>MSQHNEKNPHQHQSPLHDSSEAKPGMDSLAPEDGSHRPAAEPTPPGAQPTAPGSLKAPDTRNEKLNSLEDVRKGSENYALTTNQGVRIADDQNSLRAGSRGPTLLEDFILREKITHFDHERIPERIVHARGSAAHGYFQPYKSLSDITKADFLSDPNKITPVFVRFSTVQGGAGSADTVRDIRGFATKFYTEEGIFDLVGNNTPIFFIQDAHKFPDFVHAVKPEPHWAIPQGQSAHDTFWDYVSLQPETLHNVMWAMSDRGIPRSYRTMEGFGIHTFRLINAEGKATFVRFHWKPLAGKASLVWDEAQKLTGRDPDFHRRELWEAIEAGDFPEYELGFQLIPEEDEFKFDFDLLDPTKLIPEELVPVQRVGKMVLNRNPDNFFAENEQAAFHPGHIVPGLDFTNDPLLQGRLFSYTDTQISRLGGPNFHEIPINRPTCPYHNFQRDGMHRMGIDTNPANYEPNSINDNWPRETPPGPKRGGFESYQERVEGNKVRERSPSFGEYYSHPRLFWLSQTPFEQRHIVDGFSFELSKVVRPYIRERVVDQLAHIDLTLAQAVAKNLGIELTDDQLNITPPPDVNGLKKDPSLSLYAIPDGDVKGRVVAILLNDEVRSADLLAILKALKAKGVHAKLLYSRMGEVTADDGTVLPIAATFAGAPSLTVDAVIVPCGNIADIADNGDANYYLMEAYKHLKPIALAGDARKFKATIKIADQGEEGIV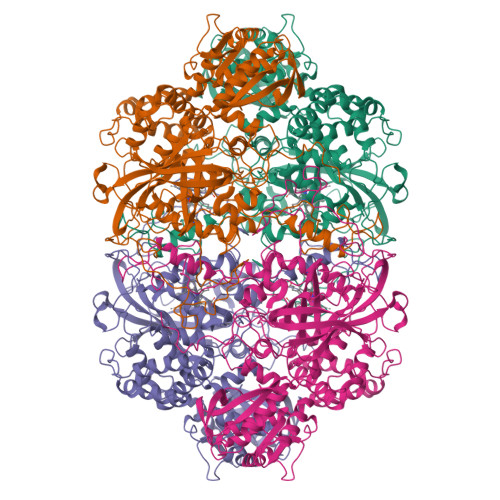EADSADGSFMDELLTLMAAHRVWSRIPKIDKIPA[4x]> QDNSRYTHFLTQHYDAKPQGRDDRYCENIMRRRGLTSPCKDINTFIHGNKRSIKAICENKNGNPHRENLRISKSSFQVTTCKLHGGSPWPPCQYRATAGFRNVVVACENGLP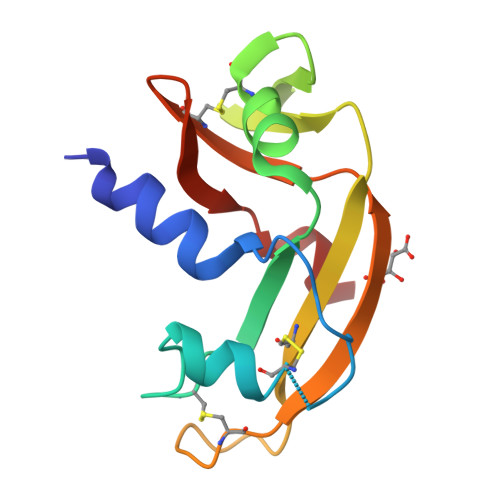VHLDQSIFRRP>HHHMFNQVMLVGRLTKDPDLRYTSAGAAVAHVTLAVNRSFKNASGEIEADYVNCTLWRKTAENTALYCQKGSLVGVSGRIQTRSYENEEGVNVYVTEVLADTVRF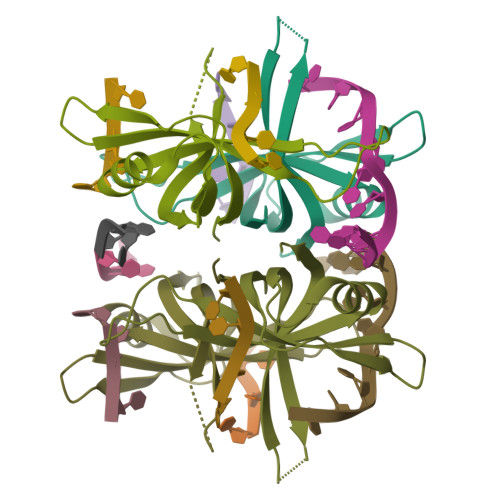MDPKPREKAAD[2x]> GSMKTNLKGETALHRACINNQVEKLILLLSLPGIDINVKDNAGWTPLHEACNYGNTVCVQEILQRCPEVDLLTQVDGVTPLHDALSNGHVEIGKLLLQHGGPVLLQQRNAKGELPLDYVVSPQIKEELFAITKIED;> GLGKGGAKRHRKVLRDN

SMC5/6 localization factor 1 (SLF1), and its interaction partner SLF2, have been identified in multiple independent proteomic analyses as proteins that accumulate at stalled replication forks with early repair factors, as part of a RAD18-SLF1-SLF2-SMC5/6 genome stability pathway. SLF1 is a 121 kDa protein containing a tandem BRCA1 C-terminal (tBRCT) domain at its N-terminus and a C-terminal Nse5-like protein domain split by an ankyrin repeat domain (ARD). Based on the high sequence similarity of this ARD to the ARD of two other DNA repair proteins, TONSL (Tonsoku-like protein) and BARD1 (BRCA1 associated RING Domain 1), the C-terminal ARD of SLF1 has been implicated in recognition of nucleosomes harbouring H4 unmethylated at K20, a characteristic of nascent nucleosomes incorporated during S phase. Our study focuses on SLF1, a multi-domain DDR protein that emerged as an essential component of the RAD18–SLF1–SLF2–SMC5/6 pathway which accumulates at stalled replication forks to facilitate efficient replication-coupled DNA repair.

To experimentally validate the interaction between SLF1 and H4 at the atomic level, we have crystallized the SLF1-H4 complex, comprising the recombinantly expressed ARD of SLF1 (SLF1ARD, residues 802-934) and a synthetic peptide of H4 N-terminal tail (H4peptide, residues 9-25). The crystal structure of SLF1ARD-H4peptide was determined by molecular replacement at 1.28 Å resolution, revealing the structure of SLF1ARD and its interface with H4. SLF1ARD contains four ankyrin repeats (labelled as ANK1-4 in Figure 1C and D), each containing a typical helix-turn-helix fold, with loops connecting consecutive repeats. The overall structure of SLF1ARD is concave in shape, like a ‘cupped hand’, as described for many other ARD structures. The well-defined extended β loop structures form the ‘fingers’ (labelled Finger 0-3), and four pairs of stacking helices form the ‘palm’. The inner surface, formed by the first helices from each ANK (labelled as αA1, αB1, αC1, and αD1 in Figure 1C and Supplementary Figure S2B), creates a negatively charged binding cavity. The H4 peptide is held by this ‘cupped hand’ with a calculated interaction surface area of 589 Å2, predominantly involving ANK1-3. SLF1ARD interacts mainly with H4 residues R17, H18, R19, and K20me0. R17 mediates a polar interaction with N850SLF1 (right top), while H18 and K20me0 bind within an acidic cavity formed by SLF1 residues D881, N850, E847, W842, D838 and E808, with H18 forming a π-π stacking interaction with W842SLF1 and a hydrogen bond with D881SLF1 (right bottom). R19 forms a hydrogen bond with the indole ring of W842SLF1 and a salt bridge with D874SLF1 outside the central binding cavity (left bottom). Importantly, K20me0 facilitates a stable interaction with SLF1 by forming salt bridges with D838, E808, and E847, explaining why unmethylated K20 is critical for recruiting SLF1 to nucleosomes (right bottom).>HATAIVTNVKHFGGMGSALRLSEAGHT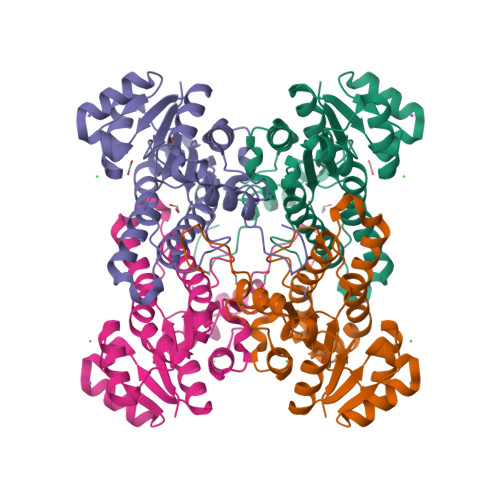VLCHDESFKQKKELEAFAETYPQLKPMSEQEPAELIRAVTRAYGQVDVLVSNDIFAPEFRPIDKYTVEDYRGAVEALQIRPFALVNAVASQMKKRKSGHIIFITSATPFGPWKELSTYTSARAGANTLANVLSKELGEYNIPVFAIGPNYLHSEDSPYFYPTTPWKTNPKHIAHVKKVTALQRLGTQKELGELVAFLASGSCDYLTGQIFWLAGGFPMIERWPGMPE[2x]>[2x]MATNNNQIGENKEQTIFDHKGNVIKTEDREIQIISKFE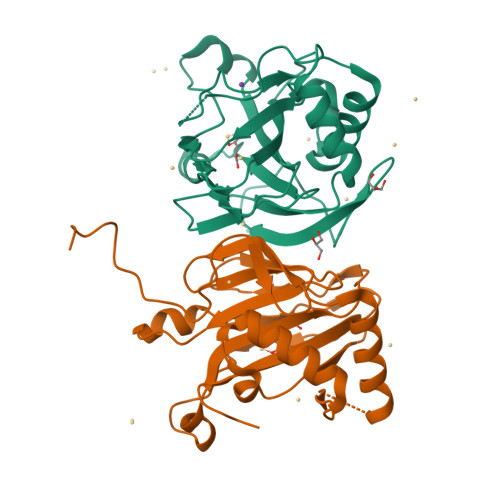EPLIVVLGNVLSDEECDELIELSKSKLARSKVGSSRDVNDIRTSSGAFLDDNELTAKIEKRISSIMNVPASHGEGLHILNYEVDQQYKAHYDYFAEHSRSAANNRISTLVMYLNDVEEGGETFFPKLNLSVHPRKGMAVYFEYFYQDQSLNELTLHGGAPVTKGEKWIATQWVRRGTYK> MSAKPQPIAAANWKCNGTTASIEKLVQVFNEHTISHDVQCVVAPTFVHIPLVQAKLRNPKYVISAENAIAKSGAFTGEVSMPILKDIGVHWVILGHSERRTYYGETDEIVAQKVSEACKQGFMVIACIGETLQQREANQTAKVVLSQTSAIAAKLTKDAWNQVVLAYEPVWAIGTGKVATPEQAQEVHLLLRKWVSENIGTDVAAKLRILYGGSVNAANAATLYAKPDIN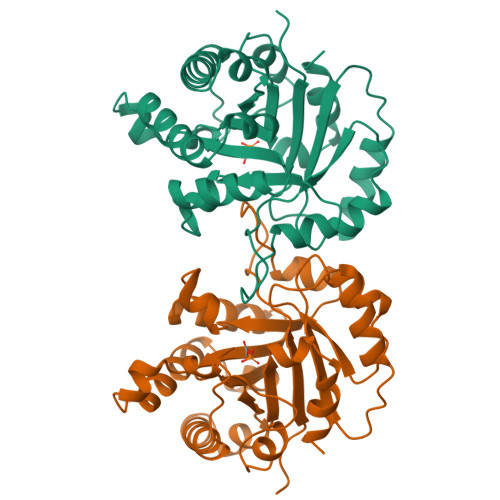GFLVGGASLKPEFRDIIDATR>[2x]MTHQTHTIAESNNFIVLDKYIKAEPTGDSYQSESDLERELIQDLRNQGYEFISVKSQSAMLANVREQLQNLNGVVFNDSEWRRFTEQYLDNPSDGILDKTRKIHIDYICDFIFDDERLENIYLIDKKNLMRNKVQIIQQFEQAGSHA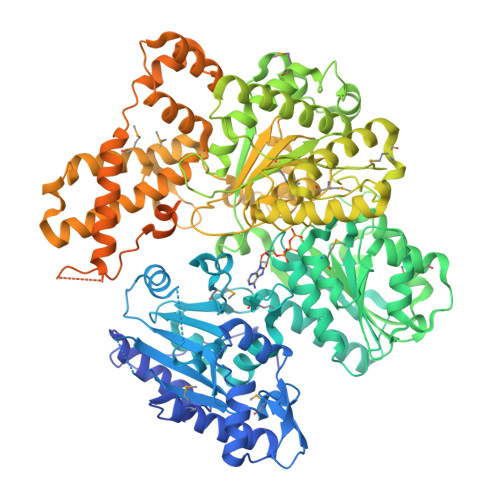NRYDVTILVNGLPLVQIELKKRGVAIREAFNQIHRYSKESFNSENSLFKYLQLFVISNGTDTRYFANTTKRDKNSFDFTMNWAKSDNTLIKDLKDFTATCFQKHTLLNVLVNYSVFDSSQTLLVMRPYQIAATERILWKIKSSFTAKNWSKPESGGYIWHTTGSGKTLTSFKAARLATELDFIDKVFFVVDRKDLDYQTMKEYQRFSPDSVNGSENTAGLKRNLDKDDNKIIVTTIQKLNNLMKAESDLPVYNQQVVFIFDECHRSQFGEAQKNLKKKFKRYYQFGFTGTPIFPENALGSETTASVFGRELHSYVITDAIRDEKVLKFKVDYNDVRPQFKSLETETDEKKLSAAENQQAFLHPMRIQEITQYILNNFRQKTHRTFPGSKGFNAMLAVSSVDAAKAYYATFKRLQEEAANKSATYKPLRIATIFSFAANEEQNAIGEISDETFDTSAMDSSAKEFLDAAIREYNSHFKTNFSTDSNGFQNYYRDLAQRVKNQDIDLLIVVGMFLTGFDAPTLNTLFVDKNLRYHGLMQAFSRTNRIYDATKTFGNIVTFRDLERSTIDAITLFGDKNTKNVVLEKSYTEYMEGFTDAATGEAKRGFMTVVSELEQRFPDPTSIESEKEKKDFVKLFGEYLRAENILQNYDEFATLKALQQIDLSDPVAVEKFKAEHYVDDEKFAELQTIRLPADRKIQDYRSAYNDIRDWQRREKEAEKKEKSTTDWDDVVFEVDLLKSQEINLDYILGLIFEHNRQNKGKGEMIEEVKRLIRSSLGNRAKEGLVVDFIQQTNLDDLPDKASIIDAFFTFAQREQQREAEALIKEENLNEDAAKRYIRTSLKREYATENGTELNETLPKLSPLNPQYKTKKQAVFQKIVSFIEKFKGVGGKI> AYGDYPNYPEGRPLFLPEAERFGNPPDLPSLLLQQRVIYISMPFLPSVTELVVAQCYYLDFDDR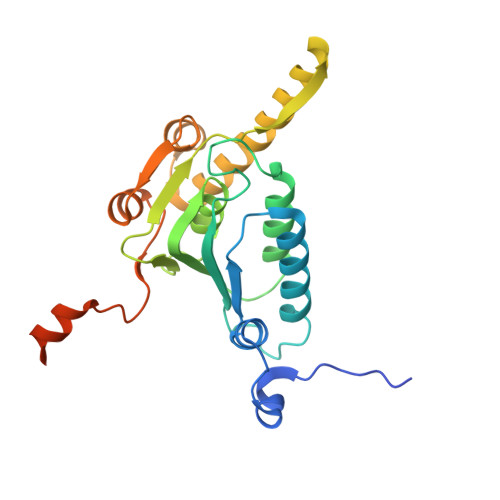NRQRPIYVYLNSTGCINDKGQAISADNEFYAIWAALGFTRAPLYTGVTWKAQNQAAVLLSAGQKGHRYSFPHAKISTAPPVMNRVFGQAVDAQLQANELDYATKYYAAILARSTGKDLETCQKQYLSRKRYFSVKEAYEEGLVDKLVPGFMLNRFRKMQKDAGVGEEDLFDMNKPKFKFRRQ>[7x]GAM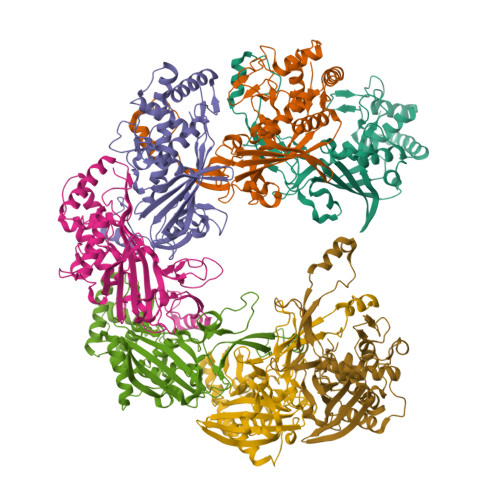SEEKNLKTASVLSFERKLDPSDALFFSGNWSNKSDDKAWQPIHLREKSVRGTISNRLKKGEADPAKLNAAIEKPNLQTVDVATLPFDSDTLKVEFTLRVLGGVGEPAACNSMEYRSKLVATISHYIDTHGLDILGNRYAANLANGRFLWRNRLGADAISIQITRLSGDESTLVGVFDALAHPLRQFEEKSVSEELEALAKLITAGLAGQEHVLLRVKAFIRMGEGQEVFPSQELLLDKGKSTKSRFLYSVGQDEKAIAAIHSQKIGNALRTIDTWYPDAEINGPIAVEPYGSVTTQGVAYRQPKAKKDFYSLLDAWVLKDKEPTIEDQHFVAAVLVRGGVFGDAS>AGDIEAGKAKAAVCAACHGQNGISQVPIYPNLAGQKEQYLVAALKAYKAGQRQGGQAPVMQGQATALSDADIANLAAYYASNPAAAA[8x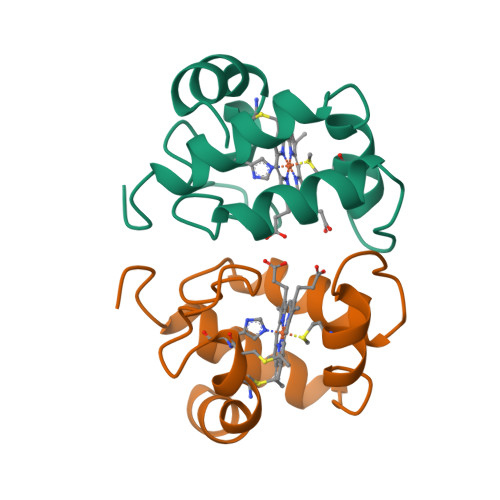]> TIHQHVDESQSSLHHTEKQIQTFITQHNNSFQELDLTNHHDVTATKRELLKLIHQQPATLYYELS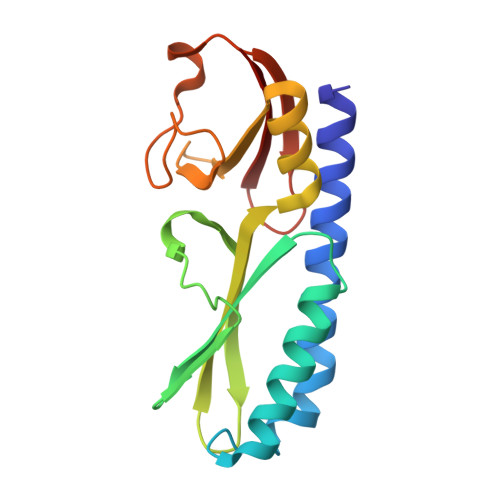GPNQFITNNYEHLNTKNMYLFSTHQLKFKNSTYMLKIYMANTPRLSEIKKDNRQFALIVDQYDNILYANDDRFTIGEKYRPQQFGFMNESVKLNHADHRLIIYKDI> KYPRPHKKLKQLHWEKLDCTDNSIWGTGKAEKFADDLYEKGVLADLEKAFAAREIKSLASKRKEDLQKITFLSRDISQQFGINLHMYSSLSVADLVKKILNCDRDFLQTPSVVEFLSKSEIIEVSVNLARNYAPYSTDWEGVRNLEDAKPPEKDPNDLQRADQIYLQLMVNLESYWGSRMRALTVVTSYEREYNELLAKLRKVDKAVSALQESDNLRNVFNVILAVGNFMNDTSKQAQGFKLSTLQRLTFIKDTTNSMTFLNYVEKIVRLNYPSFNDFLSELEPVLDVVKVSIEQLVNDCKDFSQSIVNVERSVEIGNLSDSSKFHPLDKV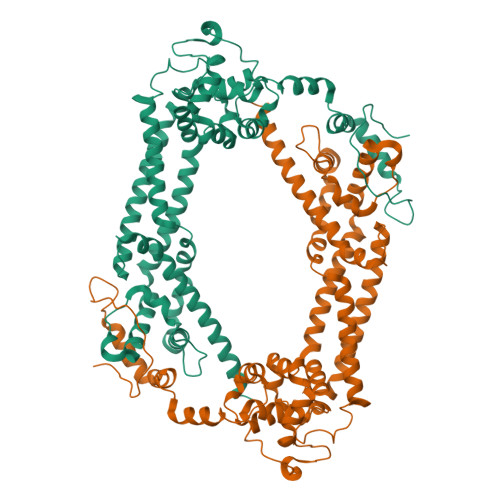LIKTLPVLPEARKKGDLLEDEVKLTIMEFESLMHTYGEDSGDKFAKISFFKKFADFINEYKKAQAQNLAAEEEERLYIKH> PQIAAHVISEASSKTTSVLQWAEKGYYTMSNNLVTLENGKQLTVKRQGLYYIYAQVTFCSNREASSQAPFIASLCLKSPGRFERILLRAANTHSSAKPCGQQSIHLGGVFELQPGASVFVNVTDPSQVSHGTGFTSFGLLKL;> AIEVKDVTDTTALITWSDDFGEYVWCELTYGIKDVPGDRTTIDLWYH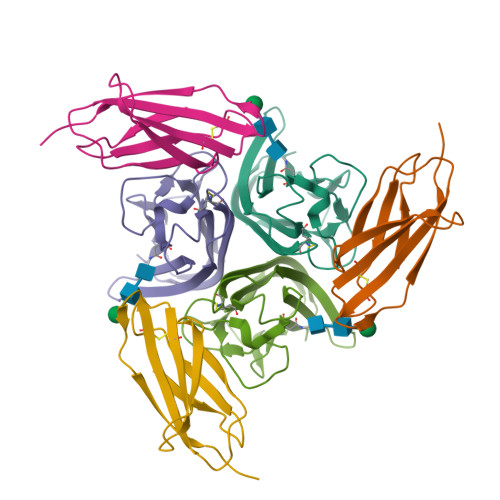HAHYSIGNLKPDTEYEVSLICRRGDMSSNPAKETFTTGLV KSHV encoded multifunctional protein ORF57 plays a key role in promoting viral mRNA accumulation and translation. Previous biochemical studies showed that ORF57 is stabilized by dimerization, which is critical for its function. ORF57 comprises of two domains with distinct putative structures: the highly disordered N-terminal domain (NTD) from residue 1 to 166, and the helix-rich C-terminal domain (CTD) from residue 167 to 455. Each monomer contains a zinc ion chelated by four residues, the cysteines at the position 333, 427, 432, and the histidine at 423, which form a consensus zinc-binding motif.

Two kinds of ORF57 crystals obtained in our experiments were used to collect X-ray diffraction data separately. The spindle-shaped crystal crystallized in the reservoir contains 0.8 M Li2SO4, 0.1 M BIS-TRIS propane and other crystallized conditions shown in Table 1. After data calculation, the cubic crystal consists only of monomers in the crystal asymmetric unit, while in the spindle shape crystal ORF57-CTD forms a dimer in the crystal asymmetric unit and the resolution was relatively lower. The dimeric crystal belongs to space group P6422 and the final structure was refined at resolution of 3.5 Å with R and Rfree values to 25.9% and 30.6%, respectively. Moreover, in the dimeric structure, only residues V168-L175 and S455 are unidentified because of the poor densities. The two monomers in the dimeric structure are nearly identical, and the root-mean-square deviation (RMSD) of atomic positions is only 0.528 Å when superimposed, but the N-terminus of the monomeric ORF57-CTD in dimer extends out to a different direction from the N-terminus of monomer if superimposed. The dimeric structure is formed by the extended N-terminal “arm” region contacting with the globular domain of the neighboring monomer and shaping as a coffee bean conformation with approximate dimensions of 69.0 × 50.9 × 50.0 Å in the asymmetric unit, with a deep groove extends around the interface of the two globular domains. The N-terminal “arm” region of one monomer protrudes out on the globular domain of another anti-parallel monomer, while the C-terminal end is enclosed into the globular domain of the same monomer. The arm extends from the globular domain of the same monomer to dock in a canyon on the surface of the globular domain of the neighboring monomer like a barb. Thus, the arm region in the dimeric structure lacks two unstable small η-helixes. PDBePISA analysis by comparing with other interactions at the dimer interface showed that the “arm” region makes major contributions, mainly (>75%) by its hydrophobic residues, suggesting the “arm” region very likely participating the dimerization.

>[2x]VSDAVKKLRLPASMIIDGESPRFDDSIIPRHHGACFNVFIPAPPSHVPEVFTDRDITALIRAGGKDDELINKKISAKKIDHLHRQMLSFVTSRHNQAYWVSCRRETAAAGGLQTLGAFVEEQMTWAQTVVRHGGWFDEKDIDIILDTAIFVCNAFVTRFRLLHLSCVFDKQSELALIKQVAYLVAMGNRLVEACNLLGEVKLNFRGGLLLAFVLTIPGMQSRRSISARGQELFRTLLEYYRPGDVMGLLNVIVMEHHSLCRNSECAAATRAAMGSAKFNKGLFFYPLS> RPSGRKSSKMQAFRIWDVNQKTFYLRNNQLVAGYLQGPNVNLEEKIDVVPIEPHALFLGIHGGKMCLSCVKSGDETRLQLEAVNITDLSENRKQDKRFAFIRSDSGPTTSFESAACPGWFLCTAMEADQPVSLTNMPDEGVMVTKFYFQEDE;> LEADKCKEREEKIILVSSANEIDVRPCPLNPNEHKGTITWYKDDSKTPVSTEQASRIHQHKEKLWFVPAKVED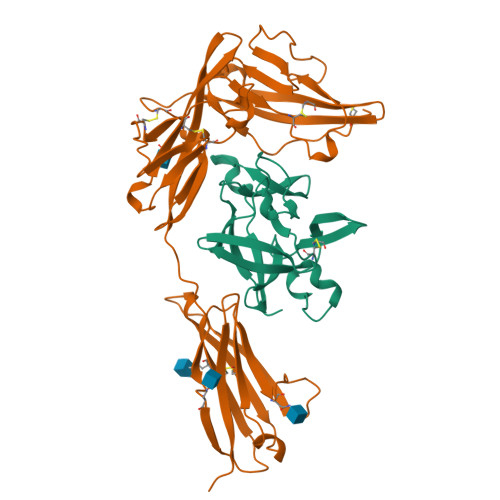SGHYYCVVRNSSYCLRIKISAKFVENEPNLCYNAQAIFKQKLPVAGDGGLVCPYMEFFKNENNELPKLQWYKDCKPLLLDNIHFSGVKDRLIVMNVAEKHRGNYTCHASYTYLGKQYPITRVIEFITLEENKPTRPVIVSPANETMEVDLGSQIQLICNVTGQLSDIAYWKWNGSVIDEDDPVLGEDYYSVENPANKRRSTLITVLNISEIESRFYKHPFTCFAKNTHGIDAAYIQLIYPVTNFQK>[9x]MCPKDWEFY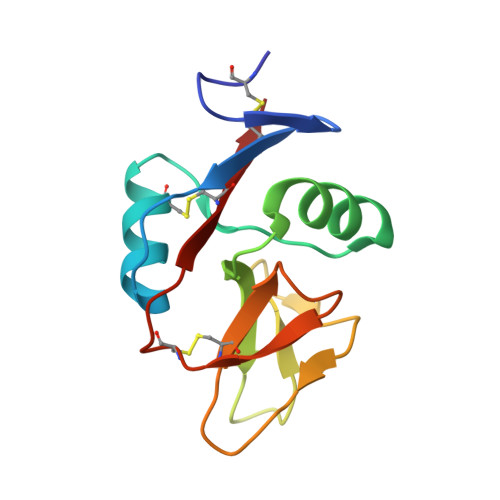QARCFFLSTSESSWNESRDFCKGKGSTLAIVNTPEKLKFLQDITDAEKYFIGLIYHREEKRWRWINNSVFNGNVTNQNQNFNCATIGLTKTFDAASCDISYRRICEKNA> MAKKNKMKPRELREAQKKARQLKAAEINNNAAPAIAAMPAAEVIAPVAEKKKSSVKAAGMKSILVSENKMYITSFGKGNSAVLEYEVDNNDYNKTQLSSKDNSNIELGDVNEVNITFSSKHGFGSGVEINTSNPTHRSGESSPVRGDMLGLKSELEKRFFGKTFDDNIHIQLIYNILDIEKILAVYVTNIVYALNNMLGIKDSESYDDFMGYLSARNTYEVFTHPDKSNLSDKVKGNIKKSLSKFNDLLKTKRLGYFGLEEPKTKDTRASEAYKKRVYHMLAIVGQIAQCVFHDKSGAKRFDLYSFINNIDPEYRDTLDYLVEERLKSINKDFIEGNKVNISLLIDMMKGYEADDIIRLYYDFIVLKSQKNLGFSIKKLREKMLEEYGFRFKDKQYDSVRSKMYKLMDFLLFCNYYRNDVAAGEALVRKLRFSMTDDEKEGIYADEAAKLWGKFRNDFENIADHMNGDVIKELGKADMDFDEKILDSEKKNASDLLYFSKMIYMLTYFLDGKEINDLLTTLISKFDNIKEFLKIMKSSAVDVECELTAGYKLFNDSQRITNELFIVKNIASMRKPAASAKLTMFRDALTILGIDDNITDDRISEILKLKEKGKGIHGLRNFITNNVIESSRFVYLIKYANAQKIREVAKNEKVVMFVLGGIPDTQIERYYKSCVEFPDMNSSLEAKRSELARMIKNISFDDFKNVKQQAKGRENVAKERAKAVIGLYLTVMYLLVKNLVNVNARYVIAIHCLERDFGLYKEIIPELASKNLKNDYRILSQTLCELCDDRNESSNLFLKKNKRLRKCVEVDINNADSSMTRKYANCIAHLTVVRELKEYIGDIRTVDSYFSIYHYVMQRC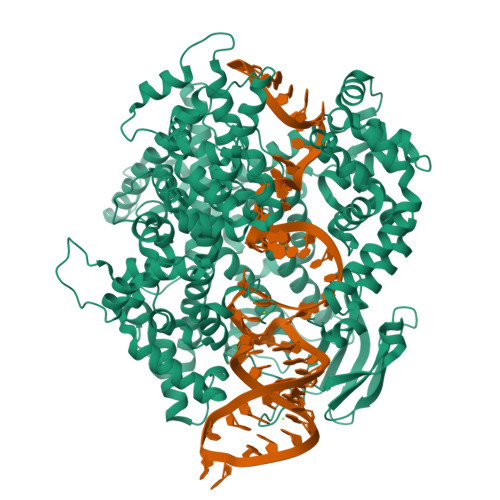ITKRGDDTKQEEKIKYEDDLLKNHGYTKDFVKALNSPFGYNIPRFKNLSIEQLFDRNEYLTEKLEHHHHHH> SGDYWLPTTMSLYQKELTDQIVSLHYSDILRYFETSHYKEDVILES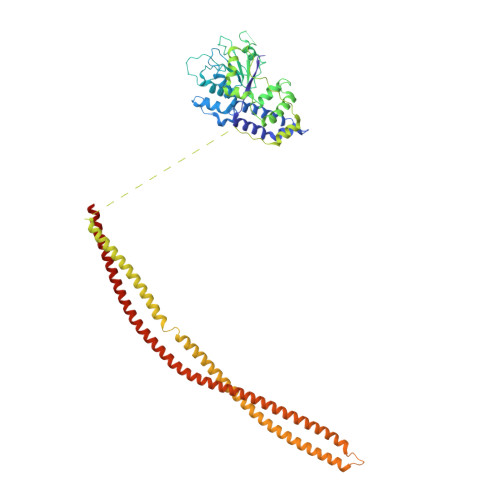MKTMCLNGSLVATHPYLLIDHYMPKSLITRDVPAHLAENSGKFSVLRDLINLVQEYETETAIVCRPGRTMDLLEALLLGNKVHIKRYDGHSIKSKQKANDFSCTVHLFSSEGINFTKYPIKSKARFDMLICLDTTVDTSQKDIQYLLQYKRERKGLERYAPIVRLVAINSIDHCRLFFGKKFDKNSREYLENVTAAMVILRDRLGTLPPDLRPIYSQKLHYLVEWLENPTVPWPLPDIYPLKQYTSMDVERSLLTEVHFKKNSSNVNYHLSSGIITHKLIQSMGEVYMDICVQKQELDDYSCLDDLQNDHLKFFSNEDEKIIKEYETVLRTNNENLNRSHELEVENNLKFSQIETLEKDIETLKGSLMAQGETLSKLKDAFVKTDNVQDEIEKEERVSVSRDTEKKYMEQEIKRAVDAIRENEEETHKLNEKQNGLESELKLKFEKSEISTKELNEKIGFLKKELKLENDLNEELVGQLSKTMDNLENLTIPRVRTQ>[4x]KELKCGSGIFITDNVHTWTEQYKFQPESPSKLASAIQKAHEEGICGIRSVTRLENLMWKQITPEL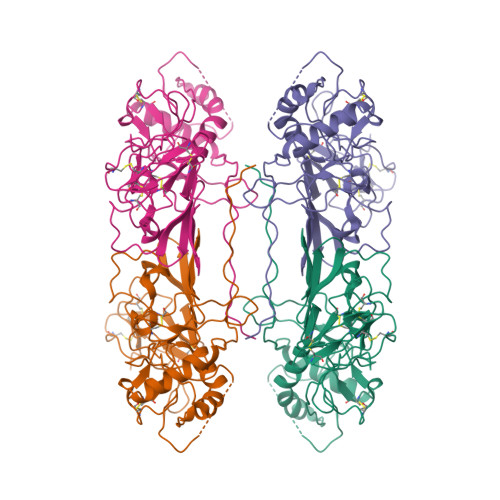NHILTENEVKLTIMTGDIKGIMQAGKRSLRPQPTELKYSWKAWGKAKMLSTELHNHTFLIDGPETAECPNTNRAWNSLEVEDYGFGVFTTNIWLKLKERQDVFCDSKLMSAAIKDNRAVHADMGYWIESALNDTWKIEKASFIEVKSCHWPKSHTLWSNGVLESEMIIPKNFAGPVSQHNYRPGYHTQTAGPWHLGRLEMDFDFCEGTTVVVTEDCGNRGPSLRTTTASGKLITEWCCRSCTLPPLRYRGEDGCWYGMEIRPLK> FYPML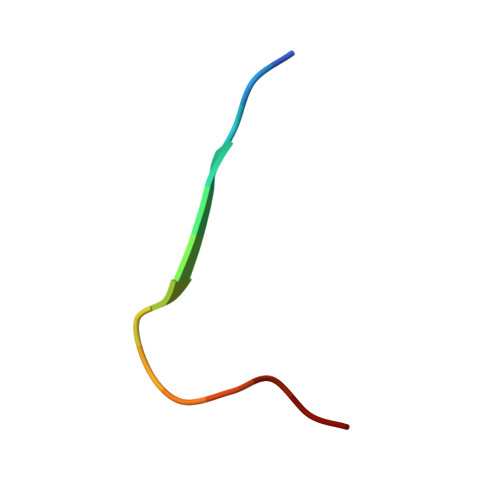RYTNGPPPT> GVSIRSMKNFYDWIKEFIRDQGEFIAQQSGWLELERSSYAKLIAQTISHVLNGGSLLVSADSSRHWFLNYILSNLNPKDLKERPL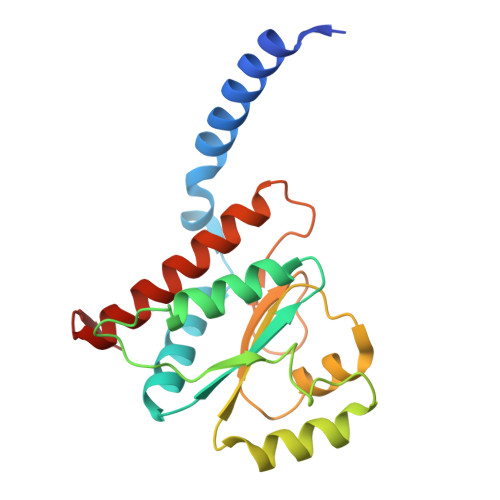LSVIDFNASSFYPKNDANLSLATIEMTYQNPMFWHVGKIENEGLKTILLSKIPSFLWLFEELKEDCLLLKEHDSLLDYKLLQLFKLFENALFSVLYNKVTL> MLVATLTLVALSAVFTNVYGSDQYTILDVYKASNVSVEDYKDLLKDLDVVHSFKVLGSSRVIFVVKMREDSYEKLSKINLPGDVYSIPAGDLSDKMQSVGVEWKRWDDLPDANLTLFERTLELKGEPLEGLASHMKAFGEKVSHVMELYPNKGFYLLGRTPPKAFVIVSLPF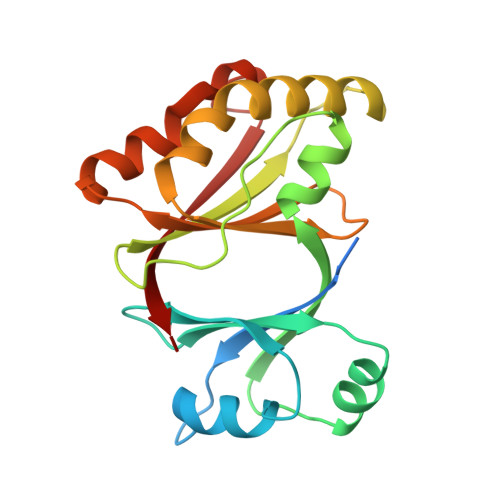RCRQVRYGSDFALNYLNGPGDSSTKVEFVAKA>[4x]MSTPGAQQVLFRTGIAAVNSTNHLRVYFQDVYGSIRESLYEGSWANGTEKNVIGNAKLGSPVAATSKELKHIRVYTL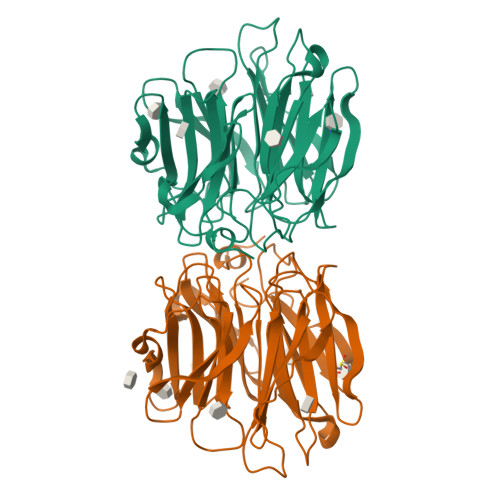TEGNTLQEFAYDSGTGWYNGGLGGAKFQVAPYSXIAAVFLAGTDALQLRIYAQKPDNTIQEYMWNGDGWKEGTNLGGALPGTGIGATSFRYTDYNGPSIRIWFQTDDLKLVQRAYDPHKGWYPDLVTIFDRAPPRTAIAATSFGAGNSSIYMRIYFVNSDNTIWQVCWDHGKGYHDKGTITPVIQGSEVAIISWGSFANNGPDLRLYFQNGTYISAVSEWVWNRAHGSQLGRSALPPA>SDLPMPM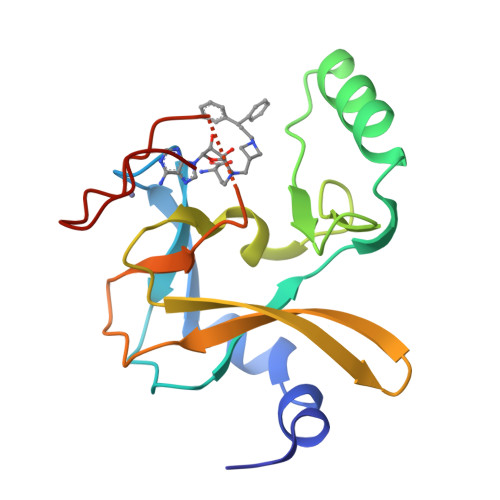RFRHLKKTSKEAVGVYRSPIHGRGLFCKRNIDAGEMVIEYAGIVIRSILTDKREKYYDSKGIGCYMFRIDDSEVVDATMHGNAARFINHSCEPNCYSRVINIDGQKHIVIFAMRKIYRGEELTYDYKFPIEDASNKLPCNCGAKKCRKFLN[2x]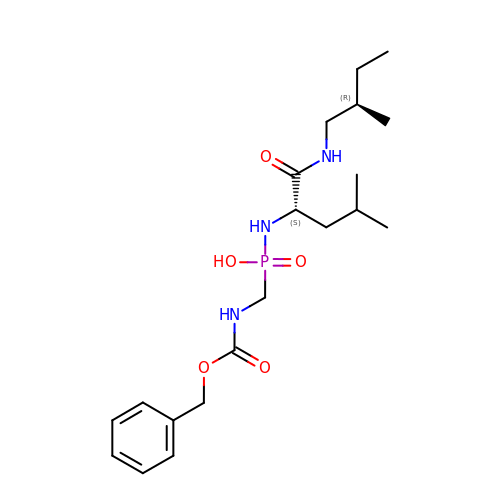P-((((benzyloxy)carbonyl)amino)methyl)-N-((S)-4-methyl-1-(((R)-2-methylbutyl)amino)-1-oxopentan- 2-yl)phosphonamidic acid | C20 H34 N3 O5 P | BHKZMZPMRWFXJX-AEFFLSMTSA-N> MGFKSWITEKLNPGQRIIRDMEPVSHRTNRKPFTTGQAYSKIEILNRTANMVIDSAAECSYTVGDKYNIVTYANGVKTKTLDTLLNVRPNPFMDISTFRRLVVTDLLFEGCAYIYWDGTSLYHVPAALMQVEADANKFIKKFIFNNQINYRVDEIIFIKDNSYVCGTNSQISGQSRVATVIDSLEKRSKMLNFKEKFLDNGTVIGLILETDEILNKKLRERKQEELQLDYNPSTGQSSVLILDGGMKAKPYSQISSFKDLDFKEDIAGFNKSICLAFGVPQVLIDGGNNANIRPNIELFYYMTIIPMLNKLTSSLTFFFGYKITPNTKEVAALTPDKEAEAKHLTSLVNNGIMTGNEARLELNLEPLDDEQMNRIRIPANVA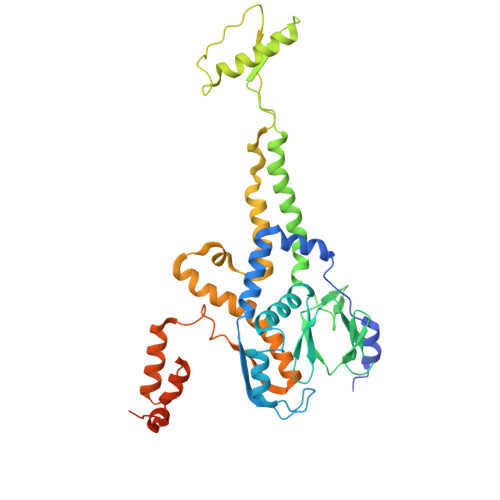GSATGVSGQEGGRPQGSTEGDKE> AKWNPAGARRPVLDEAPVFYPTEEEFEDTLKYIESIRPMAEPYGICRIVPPSSWKPPCLLKDKSIWEGSKFSTRVQKVDKLQNRKSSKKGRRGGMMKRRKLAESEENSATAHTQTGMQQSPERFGFEPGPEFTLQTFQKYADDFSKQYFRKDTSMDSVPSVEDIEGEYWRIVEV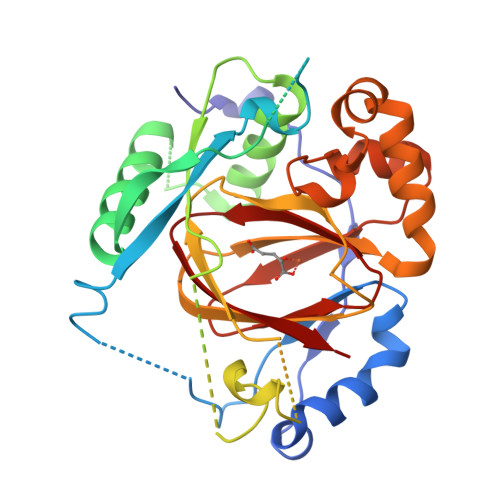PTEEIEVIYGADLETGTFGSGFPKLSPETKSDAEDKYAQSGWNLNNLPRLQGSVLSFEGGDISGVLVPWVYVGMCFSSFCWHVEDHHLYSLNYMHWGAPKLWYGVPGKDAVNLESAMRKHLPELFEEQPDLLHNLVTQFSPSLLKSEGVHVYRCVQHEGEFVLTFPRAYHAGFNCGFNCAEAVNVA> MELAEKDKGRDFTLRNARMDDIDQIIKINRLTLPENYPYYFFVEH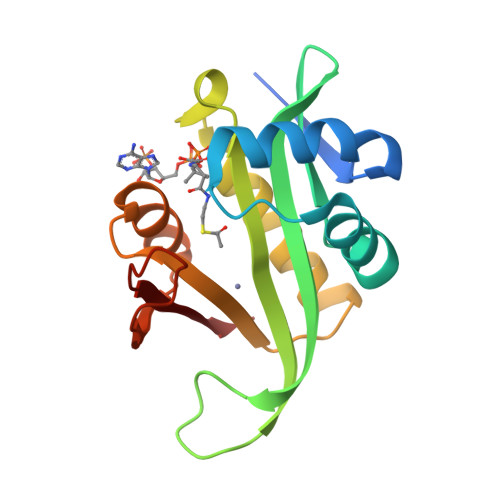LKEYGLAFFVAIVDNSVVGYIMPRIEWGFSNIKQLPSLVRKGHVVSIAVLEEYRRKGIATTLLEASMKSMKNDYNAEEIYLEVRVSNYPAIALYEKLNFKKVKVLKGYYADGEDAYLMARPL>[6x]MDWVVAPISVPENGKGPFPQRLNQLKSNKDRDTKIFYSITGPGADSPPEGVFAVEKETGW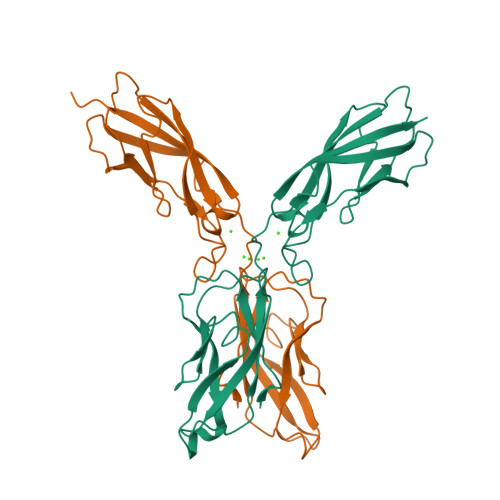LLLNKPLDREEIAKYELFGHAVSENGASVEDPMNISIIVTDQNDHKPKFTQDTFRGSVLEGVLPGTSVMQVTATDEDDAIYTYNGVVAYSIHSQEPKDPHDLMFTIHRSTGTISVISSGLDREKVPEYTLTIQATDMDGDGSTTTAVAVVEILDANDNAPMFDPQKYEAHVP> GADPVKPSRGPLVTCTCESPHCKGP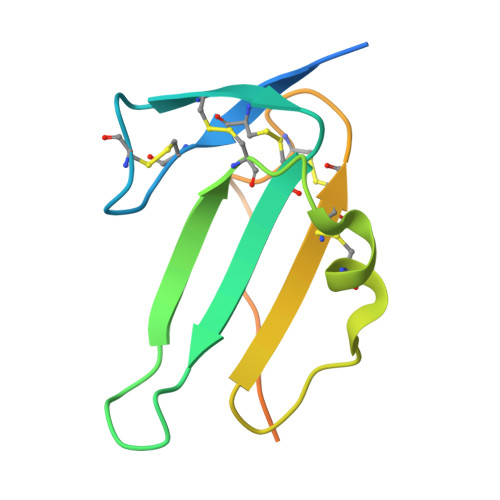TCRGAWCTVVLVREEGRHPQEHRGCGNLHRELCRGRPTEFVNHYCCDSHLCNHNVSLVLEATQPPSEQPGTDGQSGDDDDK> ARSAFSAKRSESRVPPPSDAPLPFDRVLVNEQGHYDAVTGKFTCQVPGVYYFAVHATVYRASLQFDLVKNGESIASFFQFFGGWPKPASLSGGAMVRLEPEDQVWVQVGVGDYI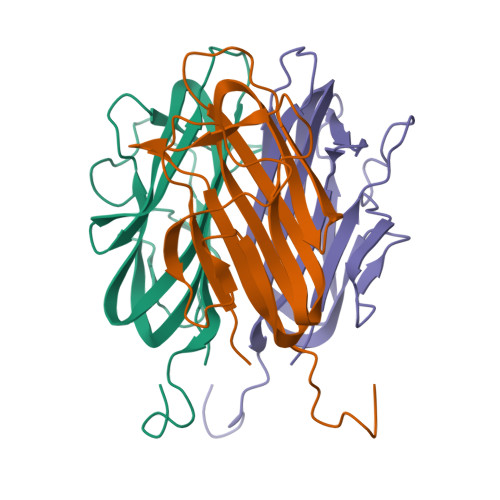GIYASIKTDSTFSGFLVYSDWHSSPVFAHHHHHH> GPGKEDRILKVWTVDPLVKVFRDSEPVTTGQALAEVARGERATLQIVIRCAKPIQELHAKVGPLALGSNAKQVLESAPVRFVGYVPVDRPIPRPPKDQLRRPPADFPDPLLEEKTIAVDENQVQPIWVTVAVPTNTQPGLYQGSVHISGRVDGRQITTKVPVAIKVFDIEVGQSRLWVTNWFSMQSRHMKIAPEPDSQQYWALLSRYARNMSEHRQNVVLVSPLSLATFQLDKSSRMEVDFSRFDRWVRIFIAEGVIGRIEGGHLGGRSSDWESPFVVRIKELREGNIITKSVAPTSEEANQFYAQFLPALVNHLRDRGWLEKYAQHLADEPVRTNIESYRAISKLVRKYAPELKIIEACHTKDLAGAIDVWVPQLNFLHNDFEHYQKRQRAGDEVWFYTCIYPQGEYANRFIEQPLLKTRLLHWINYRYGMTGYLHWGYNQWGKDSPFTHTTKQHTGQQYLPAGDPWIVYPGRDGPLDSIRHEAMCDGIADYELLSMLGERDPEAAKRLVNRHVLDFDRYNCNVEAFRATRLELLELLSRQ

Beta-N-acetylgalactosaminidases (β-NGAs) hydrolyze the different β-GalNAc linkages of various glycans to modulate the length, combination, and abundance of glycans. Despite low sequence similarity, the crystal structures of these enzymes demonstrate that all enzymes share a prototype structure and have diversified their substrate specificities (oligosaccharide-releasing, oligosaccharide/monosaccharide-releasing, and monosaccharide-releasing) through the accumulation of mutations and insertional amino acid sequences. The overall structure of these enzymes is similar to that of CpNga123 and BvGH123, which consist of a β-sandwich domain at the N-terminus and a (β/α)8-barrel domain encompassing the catalytic region. Among Groups 1–4 and GH123, the DE motif is located at the same position, suggesting that these enzymes adopt the substrate-assisted catalysis reported for GH123 MR-β-NGAs.

We used deep-sea metagenomic sequences to discover a β-NGA, NgaDssm, which is the β-NGA to possess dual OR/MR-type-β-NGA activity and low sequence similarity to known MR-β-NGAs. Assays using various pNP-substrates revealed that NgaDssm was active on GalNAc-β-pNP but not on GlcNAc-β-pNP or GalNAc-α-pNP, indicating that the enzyme possessed exo-β-NGA but not exo-β-HEX activity. Furthermore, the enzyme hydrolyzed Galβ1-3GalNAc-β-pNP but not Gal-β-pNP, demonstrating a oligosaccharide (including disaccharide)-releasing (OR)-β-NGA activity in addition to monosaccharide-releasing (MR)-type (exo-type) activity. These findings suggest that NgaDssm is an OR/MR-β-NGA. The active site of the OR/MR-type NgaDssm from Group 3 has a cleft structure that enables passage to the −2 subsites, as in NgaCa, but it also possesses two additional β-hairpins from the second and third β-sheets of the (β/α)8 barrel domain (purple). The structure of NgaDssm (Group 3) bore a striking resemblance to that of NgaLy and NgaP2 (Group 4) (root-mean-square distance of Cα atoms [rmsd] = 1.5–2.3 Å), while the structures of NgaLy and NgaP2 are identical (rmsd = 1.0 Å). The increased number of residues could potentially reinforce substrate recognition in Group 4 and GH123 enzymes. Additional structural analyses (comparison of crystal structure with AlphaFold2 predicted structure of NgaCa, comparison of apo1-form and apo2-form of NgaCa, and comparison of GalNAc-thiazoline-bond form and GlcNAc-thiazoline-/apo-form of NgaAt, NgaDssm, and NgaP2) data are illustrated in Supplementary Fig. 13. The anomeric hydrogen signal of Galβ-1-3GalNAcβ-pNP (between the GalNAc and pNP moieties) disappeared within 1 min for NgaDssm and 10 min for NgaCa and Galβ-1-3GalNAcβ appeared, while Galβ-1-3GalNAcα anomeric signals appeared after 10 and 30 min, respectively, due to mutarotation. These results indicate that NgaDssm and NgaCa are anomer-retaining enzymes, similar to GH123 enzymes.>[2x]ISEFGSSRMLTTLIYRSQVHPDRPPVDLDALVHRA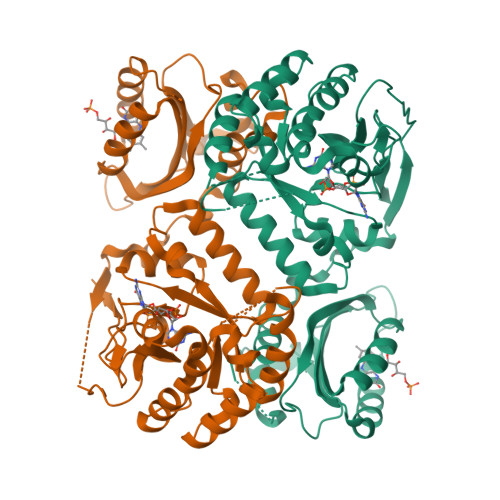SSKNLPLGITGILLFNGLQFFQVLEGTEEALESLFSEIQSDPRHRDVVELMRDYSAYRRFHGTGMRILDLRLFETDGALEEILRFSTFGVTEPVNDRMFRLLSAFIADGGRYCLPEPLQPSRWMMMPASGTAAPQHLPGQPCQFALQAIVEPAKKRVSSFEALIRSPTGGSPVEMFAAIAAEDRYRFDLESKAYAFALAGQLPLGKHQLAINLLPGSLYHHPDAVGWLMDSLLAAGLRPDQVLIEVTETEVITCFDQFRKVLKALRVAGMKLAIDDFGAGYSGLSLLTRFQPDKIKVDAELVRDIHISGTKQAIVASVVRCCEDLGITVVAEGVETLEEWCWLQSVGIRLFQGFLFSRPCLNGIGEICWPVARQAMDL> GSHMASPNGQTKPLPALKLALEYIVPAMNKHGICVVDDFLGKETGQQIGDEVRALHDTGKFTDGQLVSQKSDSSKDIRGDKITWIE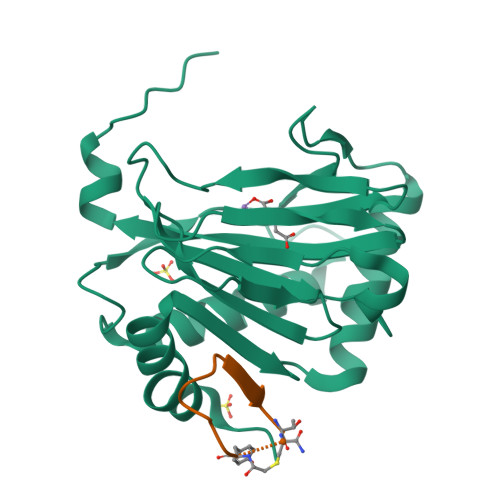GKEPGCETIGLLMSSMDDLIRHCNGKLGSYKINGRTKAMVACYPGNGTGYVRHVDNPNGDGRCVTCIYYLNKDWDAKVSGGILRIFPEGKAQFADIEPKFDRLLFFWSDRRNPHEVQPAYATRYAITVWYFDADERAAAKVKYLTGE;> XYVWLTDTWVLSRT> GSLEAQEEEEVGFPVTPQVPLRPMTYKAAVDLSHFLKEKGGLEGLIHSQRRQDILDLWIYHTQGYFPDWQNYTPGPGVRYPLTFGWCYKLVPVEPDKVEEANKGENTSLLHPVSLHGMDDPEREVLEWRFDSRLAFHHVARE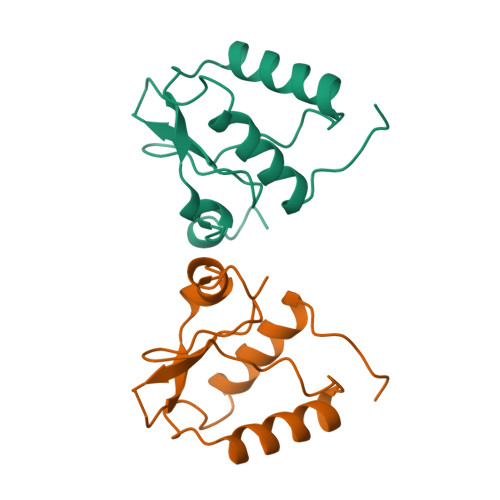LHPEYFKNC> AFKGGGPYGQGVTRGQDLSGKDFSGQTLIRQDFKTSILRQANFKGAKLLGASFFDADLTGADLSEADLRGADFSLANVTKVNLTNANLEGATMMGNTSFKGSNITGADFTDVPLRDDQRVYLCKVADGVNATTGNAT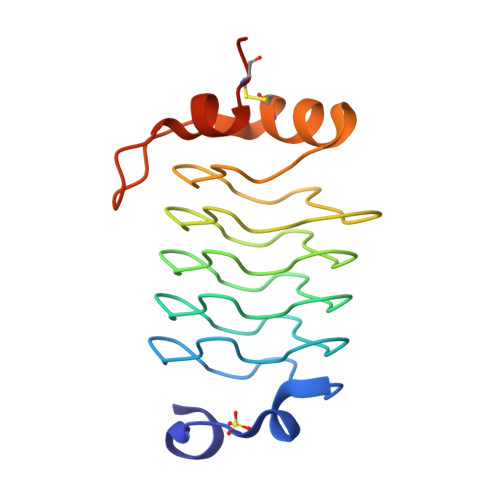RDTLLCNLEHHHHHH>MDIEFTTSAASQASLPRGRRTARPSGDDRELAILATAENLLEDRPLADISVDDLAKGAGISRPTFYFYFPSKEAVLLTLLDRVVNQADMALQTLAENPADTDRENMWRTGINVFFETFGSHKAVTRAGQAARATSVEVAELWSTFMQKWIAYTAAVIDAERDRGAAPRTLPAHEL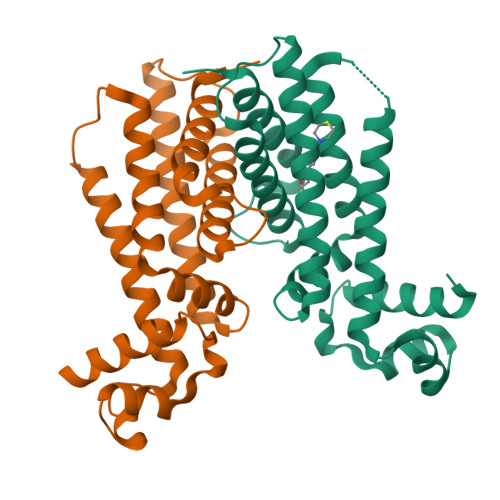ATALNLMNERTLFASFAGEQPSVPEARVLDTLVHIWVTSIYGENRGSHHHHHH[8x]> MITDCFEADIAIPSGISRPDAAALQRCEGRVVFLPTIRRQLALADVAHESFVSGGVSPDTLGLLLAYRRRFPAVITRVLPTRIVACPVDLGLTHAGTVNLRNTSPVDLCNGDPVSLVPPVFEGQATDVRLESLDLTLRFPVPLPTPLAREIVARLVARGIRDLNPD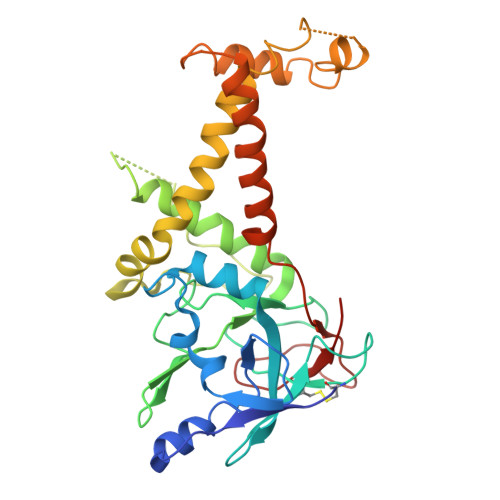PRTPGELPDLNVLYYNGARLSLVADVQQLASVNTELRSLVLNMVYSITEGTTLILTLIPRLLALSAQDGYVNALLQMQSVTREAAQLIHPEAPMLMQDGERRLPLYEALVAWLAHAGQLGDILALAPAVRVCTFDGAAVVQSGDMAPVIRYP> MSTVGSAHNVTVLGSGETTVVLGHGFGTDQSVWKYLVPHLTDDYRVLLYDNMGAGTTDPNLYDFERYSSLEGHSQDLIAILEEFHVTKCIFVGHSLSSMVGAVSSIFRPDLFRKIVMISACPRVANADDYYGGFEEEDVNQ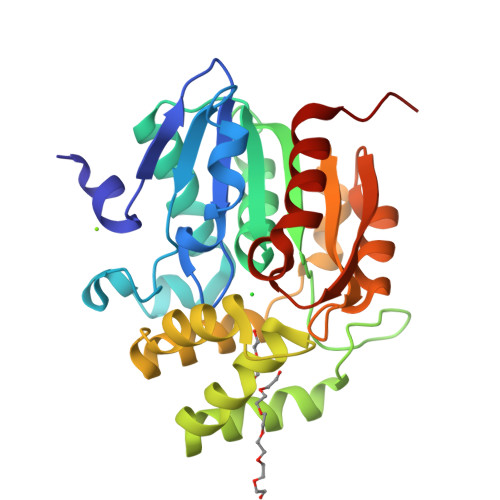LYGAMEENFQTMMTGYAPIVVGGDLESEAMQEFSRTLFNMRPDIALSICRMISGYDLRPYLGLVVIPCHIIQSSKDKLVPVAVAEYLHRNFGGKSVVELIPTEGHLPHLSAPDITIPVLIRHINQDIADD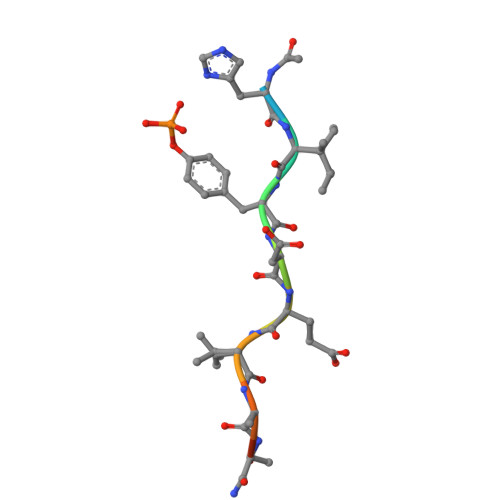> XHIYDEVAADP>MVPISPIETVPVKLKPGMDGPKVKQWPLTEEKIKALVEICTEMEKEGKISKIGPENPYNTPVFAIKKKDSTKWRKVVDFRELNKRTQDFWEVQLGIPHPAGLKQKKSVTVLDVGDAFYSVPLDKDFRKYTAFTIPSINNETPGIRYQYNVLPMGWKGSPAIFQSSMTKILEPFRKQNPDIVIYQYMDDLYVGSDLEIGQHRTKIEELRQHLLRWGFTTPDKKHQKEPPFLWMGYELHPDKWTVQPIVLPEKDSWTVNDIQKLVGKLNWASQIYAGIKVRQLSKLLRGTKALTEVVPLTEEAELELAENREILKEPVHGVYYDPSKDLIAEIQKQGQGQWTYQIYQEPFKNLKTGKYARMKGAHTNDVKQLTEAVQKIATESIVIWGKTPKFKLPIQKETWEAWWTEYWQATWIPEWEFVNTPPLVKLWYQLEKEPIIGAETFYVDGAANRETKLGKAGYVTDRGRQKVVPLTDTTNQKTELQAIHLALQDSGLEVNIVTDSQYALGIIQAQPDKSESELVSQIIEQLIKKEKVYLAWVPAHKGIGGNEQVDKLVSAG[2x];>MAHHHHHHALEVLFQGPISPIETVPVKLKPGMDGPKVKQWPLTEEKIKALVEICTEMEKEGKISKIGPENPYNTPVFAIKKKDSTKWRKLVDFRELNKRTQDFWEVQLGIPHPAGLKQKKSVTVLDVGDAYFSVPLDKDFRKYTAFTIPSINNETPGIRYQYNVLPQGWKGSPAIFQSSMTKILEPFRKQNPDIVIYQYMDDLYVGSDLEIGQHRTKIEELRQHLLRWGFTTPDKKHQKEPPFLWMGYELHPDKWTVQPIVLPEKDSWTVNDIQKLVGKLNWASQIYAGIKVRQLSKLLRGTKALTEVVPLTEEAELELAENREILKEPVHGVYYDPSKDLIAEIQKQGQGQWTYQIYQEPFKNLKTGKYARMKGAHTNDVKQLTEAVQKIATESIVIWGKTPKFKLPIQKETWEAWWTEYWQATWIPEWEFVNTPPLVKLWYQ[2x]

The structure of the N-sites of HIV-1 RT and HBV Pol are considered to be quite similar, as the amino acid sequences that form the N-sites (referred to as motifs A, B, C, D, and E) are moderately conserved in both. In our previous studies, we examined various combinations of amino acid substitutions in motifs A–E and found that the HBV-RT-associated 3MB mutant comprising Q151M in motif B and Y115F/F116Y in motif A is useful as a surrogate for structurally studying HBV RT since HIV-1 harboring RT3MB turned out to be highly sensitive against typical anti-HBV NAs, ETV, and 3TC. E-CFCP is a 4′-modified and fluoromethylenated NA that exhibits potent antiviral activity against both wild-type and drug-resistant HBVs but less potent against human immunodeficiency virus type-1 (HIV-1). The present study aimed to elucidate the mechanism of potent antiviral activity of E-CFCP against wild-type and drug-resistant HBV using HIV-1 with HBV-associated mutations in RT.

We also determined the crystal structures of HIV-1 RT3MB and RT3MB/L74V (4M) in complex with DNA and E-CFCP-TP. As a result, the structures of HIV-1 RT3MB and -RT4M complexed with DNA:E-CFCP-TP were determined at resolutions of 2.62 and 2.70 Å, respectively. The asymmetric unit of RT3MB/4M crystals contains two HIV-1 RT p66-p51 heterodimers complexed with DNA (chains ABE and CDF). Chains A and C, B and D, and E and F correspond to the p66 and p51 subunits and DNA, respectively. The clear electron density map enabled us to construct a complete atomic model of the bound E-CFCP-TP at the HIV-1 RT3MB/4M N-site in both chains A and C. Nevertheless, the average B-values of the final refined E-CFCP-TP model were relatively high (100–110 Å2) compared with those of polypeptide chains and DNA close to the N-site (~ 75 Å2). In addition, the superimposition of the four chains (chain A and C of RT3MB/4M) indicated that the bound E-CFCP-TP varied in conformation with an RMSD of ~ 0.5 Å, and the electron density peak for Mg2+ was absent in chain A of RT4M. These observations suggest that the bound E-CFCP-TP is slightly perturbed within the N-site of crystallized RT3MB/4M. The fluorine atom is located midway between the Met184 and Asp185 sidechains with interatomic distances of 3.5–4.0 Å; the fluoromethylene pushes the Met184 sidechain backward and fills the gap between the Met184 and Asp185 sidechains. The 4′-cyano exploits the deep hydrophobic pocket created by the Ala114, Phe115, Met184, Asp185, and Phe160 sidechains. Superimposition of the bound E-CFCP-TP, ETV-TP, and dGTP in HIV-1 RT3MB/4M highlights the deviated binding of the cyclopentyl moiety of E-CFCP-TP; the cyclopentyl moiety is shifted approximately 0.6 Å toward Met151 and skewed by approximately 10°.> MGHMNITDIREQFPILHQQVNGHDLVYLDSAATSQKPRAVIETLDKYYNQYNSNVHRGVHTLGTRATDGYEGAREKVRKFINAKSMAEIIFTKGTTTSLNMVALSYARANLKPGDEVVITYMEHHANIIPWQQAVKATGATLKYIPLQEDGTISLEDVRETVTSNTKIVAVSHVSNVLGTVNPIKEMAKIAHDNGAVIVVDGAQST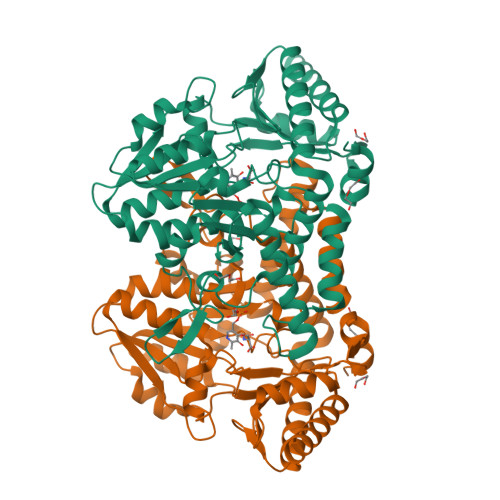PHMKIDVQDLDCDFFALSSHKMCGPTGVGVLYGKKALLENMEPAEFGGEMIDFVGLYESTWKELPWKFEAGTPIIAGAIGLGAAIDFLEEIGLDEISRHEHKLAAYALERFRQLDGVTVYGPEERAGLVTFNLDDVHPHDVATVLDAEGIAVRAGHHCAQPLMKWLDVTATARASFYLYNTEEEIDKLVEALQKTKEYFTNVFVDLEHHHHHH>[4x]SNAMSTLGTLAPAADTELFADT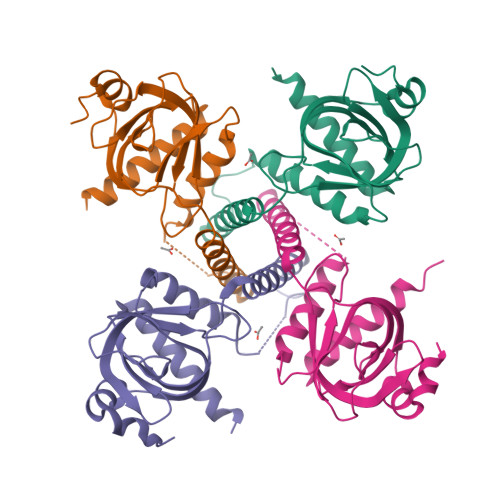LSCELRLPAGFHVTADPGSHATAETLLRSLGQVEDLRSEDSSEERGELPLLVQRMDAKLDLILALIGRLVRQSDTRLALGTVHWSVRGIRLASPHAHPPGTTGSVLLQPSDWLPELLQLPADVLASASDGQQHWLWLRFAPLGTGLQDALERHLFRLHRRQIADARRQR> MPSATPGAPAASAAMQEALEGAGRIIDRLLQEDRAYPDLSELLNVPVHTCPTISGVSEMDYPLQSPGLLTIPSLPEISAIRRVPLPPELIEQFGHMQCNCMMGVFPEISRAWLTIDSDIFMWNYEDGGDLAYYDGLSETILSVGLVKPKTGIFQPHIRFLLVLSTPVDIVILGLSFANLQPGNLNDSISGGMQLLPDPLYSLPTDNTYLLSITSTDNGRIFLSGKDGCLYEVEYQAEAGWFSQRCRKINHSKSSLSFLVPSVLQFAFSEDDPIVQIAIDNSRNILYTRSEKGVIQVYDLGVDGHGMSRVASVSQNSLVSAAGNIARTIDRNVFKPIIHISVIEMSESVNCHLLAVTHTGVRFYFSTVPFKQPTARPCMLALVHVRLPPGFSASSNVEKPSKVHKALYNNGVLLMAASENEDNDMLWCINRDSFPFQKPMMETQVTTQVDGHSWALSAVDEQKADKIVTPLNKDLIPLTDSPVIIQQHMIPPKRFVLLSAQGSHIFYKLRPVDQLRHLLVSNSGGDGEEIERFFKLHQENQACATCLILACSSAASDREVSSWAARAFFRYGGEAQLRVQSALHAPSNVGPIFGSPLPVASPIPVGSPMPNPSFLGTPTQGACPPNVSTPAYGVATPAPQPPAVPGMMGTEIVFSGKHNGICIYFCRIIGNIWDGSVAVENTFQSGNREVTAIDSSVTPQHLESVLKELKGLLEFLDRYSQFTAGSLGNPGFGTPANRQQRLVSLGRPDIGSSQQAQQELQRKYHTEAQLAEQFSLQGIHQLVRKMCQAL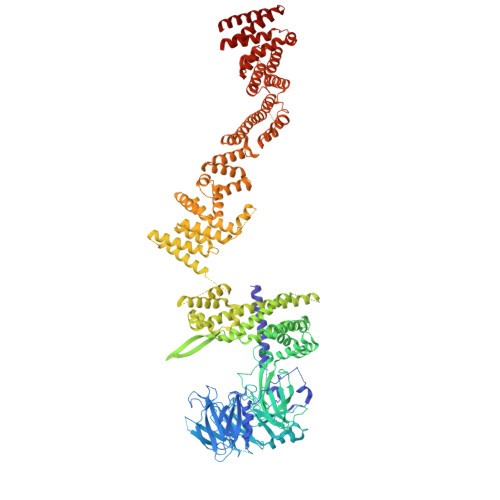ALWKLLCEHQFSLVVSDLQKELQEQLKITTFKDLVIRDKELTGALTASLISCYIRDNASVDGISYRLQEVCPLLYSTDDAVCSKANELLQRSRHVPNKQEKERMLRESLKEYQKISQQVDLPNVCAQYRQVRFYEGVVELCLSAAEKKDPQGLGLHFHKNGEPEEDMAGLQAFQERLNSYKCITDTLQELVNQSKAAPQSPSVPKKPGPPVLSSDPNMLSNEEAGIHFEQMLKLAQRSADELFNIALFNWLIQADLTDKLLELNSPFLEPHLVRMAKLDQNKVRYMDLLWRYYEKNRNFSNAARVVAKLADMHSPEISLKQRLEYISRAILSAKSSTTMSTLAADGEFLHELEEKLEVARIQLQIQETLTRQYSHHSTVGDAVSQLDSQLMDITKMFGQYADPFRLSECKLAIIHCAGHSDPILVQTLWQDIIDKELSDSMGNSSVDRMQSLHLKITSLGKIYASTPRYFPLEFLVKYLEQQVCNFSWDAGFVTYTMQEINVPVPKLLEVYDHLFKARDPWWSRMKKPLHLLESIYILLSGYVQEPSKVPSYERRRFTTLCLDAISCYLVELQSMDPAPALLNTVSNFKSLQAKLERLS In this work, we present the structural analysis of human METTL16 based on two X-ray crystal structures of the N-terminal MTase domain (residues 1–291) of human METTL16 (METTL16_291): an apo form at 1.9 Å resolution and a post-catalytic complex with S-adenosylhomocysteine (SAH) at 2.1 Å resolution. To provide structural insights into the methyltransferase reaction catalyzed by the MTase domain of METTL16, we solved X-ray crystal structures of apo and SAH-bound METTL16_291 (METTL16_291/SAH). These structures confirmed that METTL16 is a Class I SAM-MTase that uses a conserved Rossmann fold to bind the SAH product and likely SAM, the methyl-donor substrate. The conserved SAM-MTase core (residues 79–288) of METTL16_291 possesses a mostly parallel, seven-stranded β sheet (β1–β7) organized as ‘3214576’, with β7 being antiparallel. Although the MTase domain of METTL16 has a canonical Class I MTase structure, METTL16_291 has several unique structural regions: residues 1–78 that precede the Rossmann fold as well as residues 95–97 (ηZ) and 188–222 (a putative loop containing disordered residues 188–214) within the Rossmann fold.

Structural comparisons of apo and SAH-bound METTL16_291 structures revealed that the cofactor-binding site in the apo structure is occupied by four water molecules, which serve as placeholders for the following heteroatoms: (i) amino and carboxyl groups of the homocysteine moiety, (ii) 3′-hydroxyl of the ribose moiety and (iii) N1 of adenine. The β sheet appears to be stabilized by a disulfide bridge between C183 and C247, thereby linking the β4 and β5 strands. This disulfide bridge is present at approximately 40% occupancy in the apo structure and is absent in the SAH-bound complex, likely because of radiation damage and/or the presence of Tris(2-carboxyethyl)phosphine hydrochloride (TCEP) in the protein buffer. Comparison of the apo METTL16_291, SAH-bound METTL16_291, and SAH-bound METTL16_40–291 structures revealed significantly different orientations of the 184NPPFF188 motif. Additionally, the 184NPPF187 residues are adjacent to a disordered region spanning 189–213 in the apo structure and 188–214 in the SAH-bound complex; these residues could not be modeled due to a lack of electron density. This disordered segment is one of the elements that distinguishes the Rossmann fold of METTL16 from other SAM-MTases. Hence, it may play an important role in RNA substrate recognition and/or orienting molecules for catalysis.

> SNAMALSKSMHARNRYKDKPPDFAYLASKYPDFKQHVQINLNGRVSLNFKDPEAVRALTCTLLREDFGLSIDIPLERLIPTVPLRLNYIHWVEDLIGHQDSDKSTLRRGIDIGTGASCIYPLLGATLNGWYFLATEVDDMCFNYAKKNVEQNNLSDLIKVVKVPQKTLLMDALKEESEIIYDFCMCNPPFFANQLEAKGVNSRNPRRPPPSSVNTGGITEIMAEGGELEFVKRIIHDSLQLKKRLRWYSCMLGKKCSLAPLKEELRIQGVPKVTYTEFCQGRTMRWALAWSFYD>[2x]VTHKAVHEFVSGTPGKELPQEVKALLPVDQTDLKDGIQVTP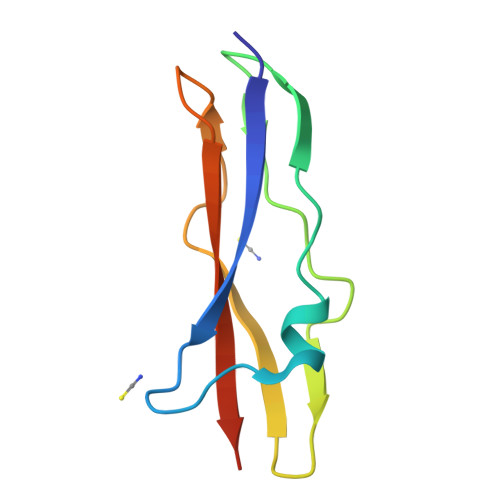TQPSQTEVKTSEGTWSFKSYDKTSETVNGSDVKFVGTWEFTASPAPT>GSHMFSLITWNIDGLDLNNLSERARGVCSYLALYSPDVIFLQEVIPPYYSYLKKRSSNY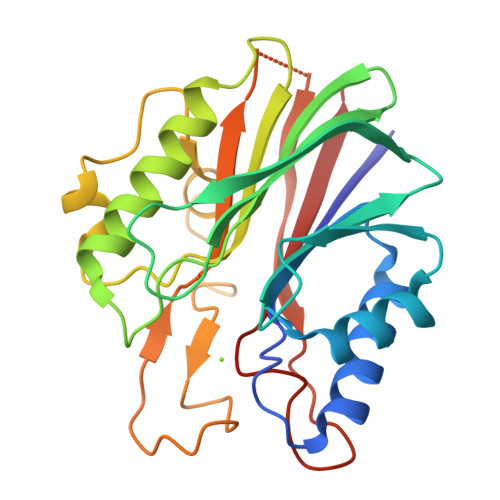EIITGHEEGYFTAIMLKKSRVKLKSQEIIPFPSTKMMRNLLCVHVNVSGNELCLMTSHLESTRGHAAERMNQLKMVLKKMQEAPESATVIFAGDTNLRDREVTRSGGLPNNIVDVWEFLGKPKHCQYTWDTQMNSNLGITAACKLRFDRIFFRAAAEEGHIIPRSLDLLGLEKLDCGRFPSDHWGLLCNLDIIL[2x]(12S)-12-methyltetradecanoic 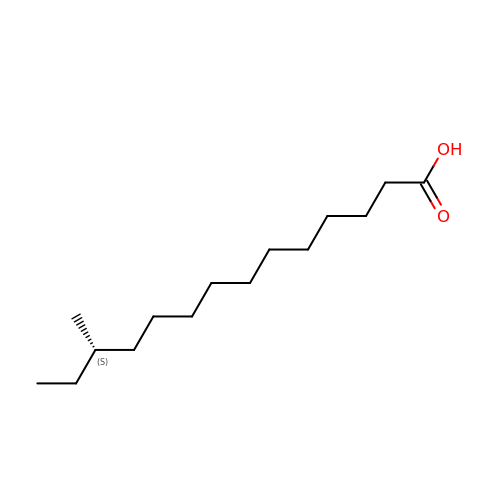acid | C15 H30 O2 | XKLJLHAPJBUBNL-AWEZNQCLSA-N> EVKLSGDARMGVMYNGDDWNFSSRSRVLFTMSGTTDSGLEFGASFKAHESVGAETGEDGTVFLSGAFGKIEMGDALGASEALFGDLYEVGYTDLDDRGGNDIPYLTGDERLTAEDNPVLLYTYSAGAFSVAASMSDGKVGETSEDDAQEMAVAAAYTFGNYTVGLGYEKIDSPDTALMADMEQLELAAIAKFGATNVKAYYADGELDRDFARAVFDLTPVAAAATAVDHKAYGLSVDSTFGATTVGGYVQVLDIDTIDDVTYYGLGASYDLGGGASI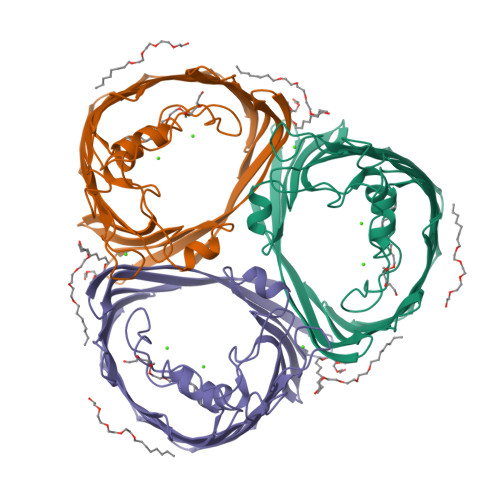VGGIADNDLPNSDMVADLGVKFKF> SMSSWKKQAEDIKKIFEFKETLGTGAFSEVVLAEEKATGKLFAVKCIPKKALKGKESSIENEIAVLRKIKHENIVALEDIYESPNHLYLVMQLVSGGELFDRIVEKGFYTEKDASTLIRQVLDAVYYLHRMGIVHRDLKPENLLYYSQDEESKIMISDFGL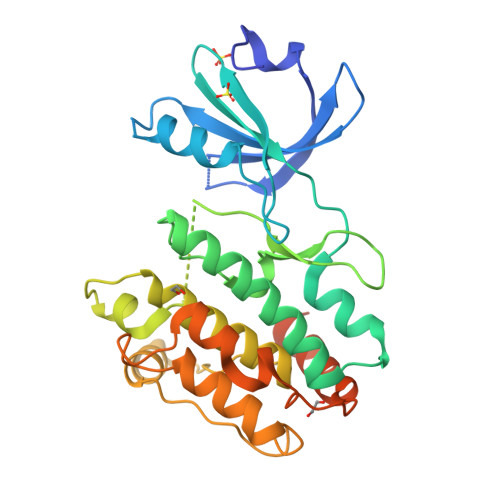SKMEGKGDVMSTACGTPGYVAPEVLAQKPYSKAVDCWSIGVIAYILLCGYPPFYDENDSKLFEQILKAEYEFDSPYWDDISDSAKDFIRNLMEKDPNKRYTCEQAARHPWIAGDTALNKNIHESVSAQIRKNFAKSKWRQAFNATAVVRHMRKLHLGSSLD>[8x]FACKTANGTAIPIGGGSANVYVNLAPVVNVGQNLVV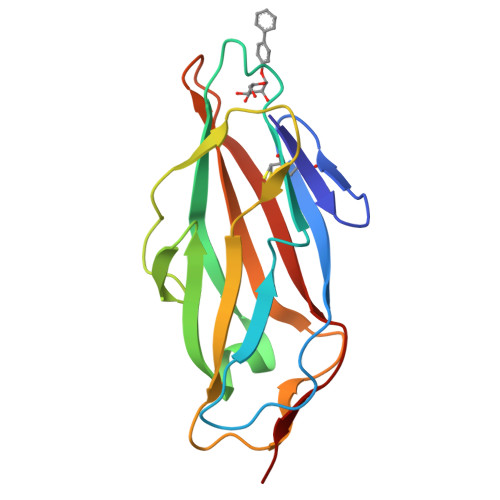DLSTQIFCHNDYPETITDYVTLQRGSAYGGVLSNFSGTVKYSGSSYPFPTTSETPRVVYNSRTDKPWPVALYLTPVSSAGGVAIKAGSLIAVLILRQTNNYNSDDFQFVWNIYANNDVVVPT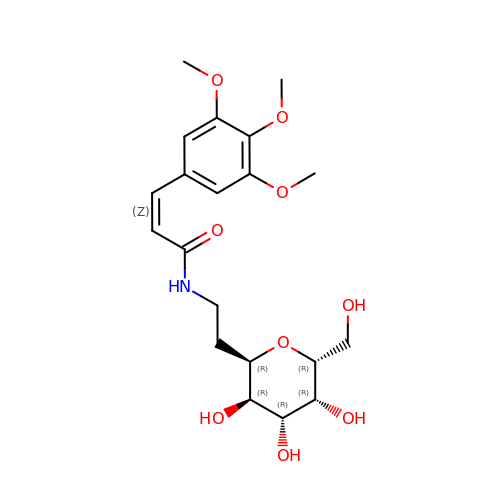(~{Z})-~{N}-[2-[(2~{R},3~{R},4~{R},5~{R},6~{R})-6-(hydroxymethyl)-3,4,5-tris(oxidanyl)oxan-2-yl]ethyl]-3-(3,4,5-trimethoxyphenyl)prop-2-enamide | C20 H29 N O9 | PZZVIPJMQGXDNG-MLJSDRKUSA-N>[6x]AKDCKRESNTFPGICITKPPC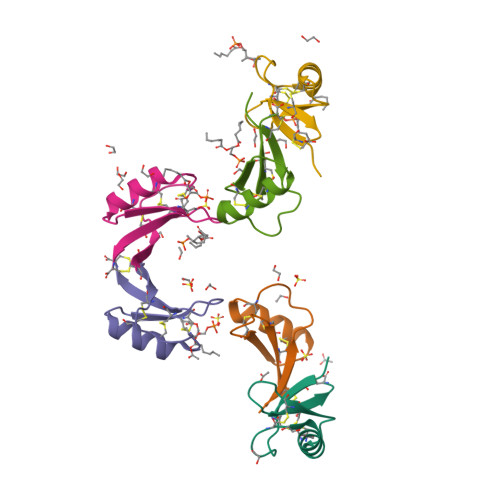RKACIREKFTDGHCSKILRRCLCTKPC hydrogen [(1S)-1-hydroxy-2-(3-octyl-1H-imidazol-3-ium-1-yl)-1-phosphonoethyl]phosphonate 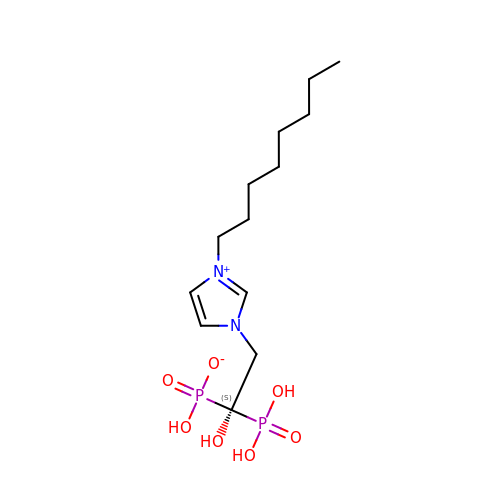| C13 H26 N2 O7 P2 | AZKPHAACXOXPFR-UHFFFAOYSA-N2-methyl-3~{H}-isoindol-1-one 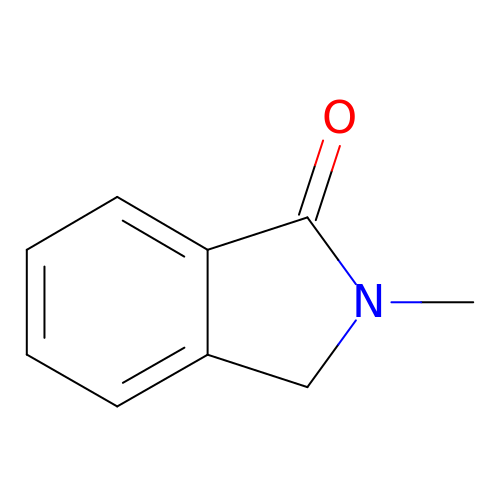| C9 H9 N O | JHMBTUMIVBSJFS-UHFFFAOYSA-N> GSHMPYTIELIQPEDGEAVIAMLKTFFFKDEPLNTFLDLGECKELEKYSLKPLPDNCSYKAV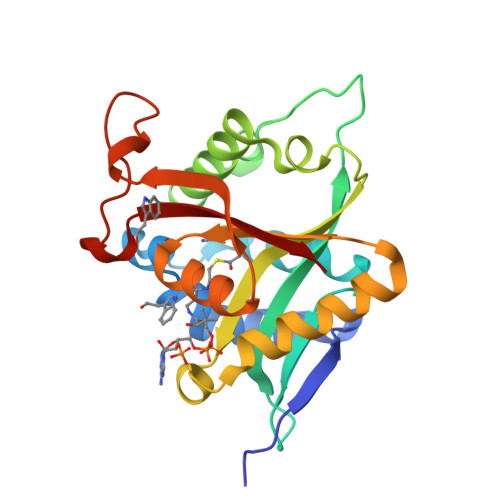NKKGEIIGVFLNGLMRRPSPDDVPEKAADSCEHPKFKKILSLMDHVEEQFNIFDVYPDEELILDGKILSVDTNYRGLGIAGRLTERAYEYMRENGINVYHVLCSSHYSARVMEKLGFHEVFRMQFADYKPQGEVVFKPAAPHVGIQVMAKEV> GSSNSQVEQILAEFQLQAADLKKVMRRMQKEMDRGLRLETHAAASVKMLPTYVRSTPEGSEVGDFLSLDLGGTNFRVMLVKVGEGEEGQWSVKTKHQMYSIPEDAMTGTAEMLFDYISECISDFLDKHQMKHKKLPLGFTFSFPVRHEDIDKGILLNWTKGFKASGAEGNNVVGLLRDAIKRRGDFEMDVVAMVNDTVATMISCYYEDHQCEVGMIVGTGCNACYMEEMQNVELVEGDEGRMCVNTEWGAFGDSGELDEFLLEYDRLVDESSANPGQQLYEKLIGG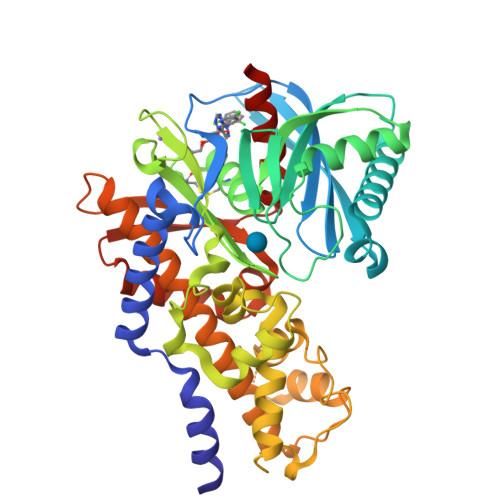KYMGELVRLVLLRLVDENLLFHGEASEQLRTRGAFETRFVSQVESDTGDRKQIYNILSTLGLRPSTTDCDIVRRACESVSTRAAHMCSAGLAGVINRMRESRSEDVMRITVGVDGSVYKLHPSFKERFHASVRRLTPSCEITFIESEEGSGRGAALVSAVACKKACMLGQ>[2x]MIDYTAAGFTLLQGAHLYAPEDRGICDVLVANGKIIAVASNIPSDIVPNCTVVDLSGQILCPGFIDQHVHLIGGGGEAGPTTRTPEVALSRLTEAGVTSVVGLLGTDSISRHPESLLAKTRALNEEGISAWMLTGAYHVPSRTITGSVEKDVAIIDRVIGVKCAISDHRSAAPDVYHLANMAAE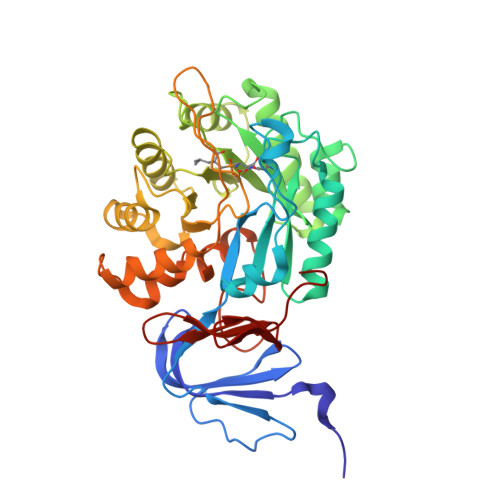SRVGGLLGGKPGVTVFHMGDSKKALQPIYDLLENCDVPISKLLPTHVNRNVPLFEQALEFARKGGTIDITSSIDEPVAPAEGIARAVQAGIPLARVTLSSDGNGSQPFFDDEGNLTHIGVAGFETLLETVQVLVKDYDFSISDALRPLTSSVAGFLNLTGKGEILPGNDADLLVMTPELRIEQVYARGKLMVKDGKACVKGTFETA> MNLVLMGLPGAGKGTQAEKIVAAYGIPHISTGDMFRAAMKEGTPLGLQAKQYMDRGDLVPDEVTIGIVRERLSKDDCQNGFLLDGFPRTV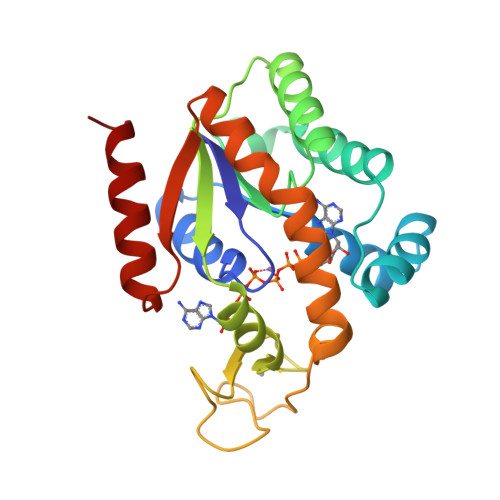AQAEALETMLADIGRKLDYVIHIDVRQDVLMERLTGRRICRNCGATYHLIFHPPAKPGVCDKCGGELYQRADDNEATVANRLEVNMKQMKPLVDFYEQKGYLRNINGEQDMEKVFADIRELLGGLAR> MENTENSVDSKSIKNLEPKIIHGSESMDSGISLDNSYKMDYPEMGLCIIINNKNFHKSTGMTSRSGTDVDAANLRETFRNLKYEVRNKNDLTREEIVELMRDVSKEDHSKRSSFVCVLLSHGEEGIIFGTNGPVDLKK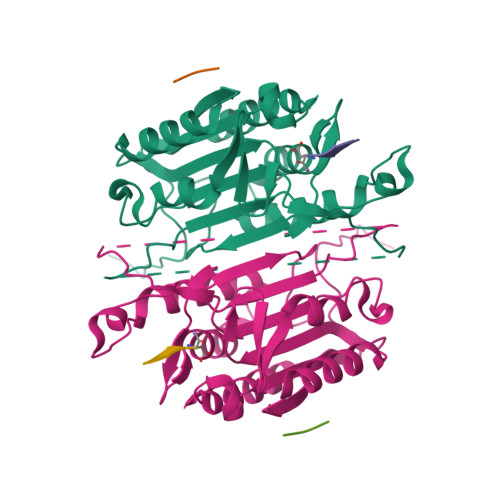ITNFFRGDRCRSLTGKPKLFIIQACRGTELDCGIETDSGVDDDMACHKIPVEADFLYAYSTAPGYYSWRNSKDGSWFIQSLCAMLKQYADKLEFMHILTRVNRKVATEFESFSFDATFHAKKQIPCINSMLTKELYFYHL;> LSS Breakdown is then initiated with the conversion of the C‐3 hydroxyl group to a ketone (cholest‐4‐en‐3‐one, cholestenone) by the oxidase ChoD, and further oxidation at the C‐26 “tail” region via a three‐step process involving oxidation to the hydroxyl, aldehyde, and carboxylic acid species. These sidechain‐modifying reactions are catalysed by the cytochromes P450 CYP125A1 and CYP142A1 (CYP125 and CYP142 hereafter). Comparison of the effect of complementing a CYP125 knockout in the CDC1551 strain of Mtb (which does not express the CYP142 protein), with CYP125 or CYP142 reveals that the two enzymes are functionally redundant with respect to growth on cholesterol. Here we present a series of compounds based on an ethyl 5‐(pyridin‐4‐yl)‐1H‐indole‐2‐carboxylate pharmacophore which bind strongly to both Mtb cholesterol oxidases CYP125 and CYP142.

The introduction of a methylenecyclohexyl group on the indole NH, compound 7, maintained affinity with both CYP125 and CYP142. Upon inspection of the corresponding CYP125 ligand complex X‐ray crystals structures, it was noted that elaboration from the R1 position (N of the indole) dramatically changes the binding pose of this series. In the cases of compounds 7, 8, 10, and 12 the ligand is observed at a greater distance from the heme, typically with the pyridine coordination mediated via a water molecule, to produce a reverse‐type I interaction similar to what was observed for the inhibitor LP10. In the case of compounds 7 and 8, which feature an aliphatic ring on a methylene linker, it appears that movement of the compound deeper into the active site is blocked by Phe100, leading to a distance of 3.9 Å and 3.3 Å, respectively between the pyridine nitrogen and the heme distal water molecule. R1 position are observed significantly closer to the heme iron, with compound 10 observed at 2.4 Å from the distal water. This is likely attributable to the ability of the additional carbon to facilitate positioning of the ring closer to the plane of the indole, as opposed to compounds 7 and 8 which extend at an angle of 67° from this plane because of the geometric requirements of the single carbon linker. In the crystal structures of CYP125 in complex with 7 and 8, Ile97 and Phe100, which form part of the loop preceding the B’ helix, are positioned below the R1 ring structures seemingly blocking further ingress of the compounds. In the same structures, Thr201, which is found in the loop preceding the F α‐helix is observed in a different conformation relative to that which is observed for compound 4, forming a hydrogen bond with the sidechain of Glu271 and further restricting any downward movement of the compound.

> NGPSPNLPPGFDFTDPAIYAERLPVAEFAELRSAAPIWWNGQDPGKGGGFHDGGFWAITKLNDVKEISRHSDVFSSYENGVIPRFKNDIAREDIEVQRFVMLNMDAPHHTRLRKIISRGFTPRAVGRLHDELQERAQAIAAEAAAAGSGDFVEQVSCELPLQAIAGLLGVPQEDRGKLFHWSNEMTGNEDPEYAHIDPKASSAELIGYAMKMAEEKAKNPADDIVTQLIQADIDGEKLSDDEFGFFVVMLAVAGNETTRNSITQGMMAFAEHPDQWELYKKVRPETAADEIVRWATPVTAFQRTALRDYELSGVQIAAGQRVVMFYRSANFDEEVFQDPFTFNILRNPNPHVGFGGTGAHYCIGANLARMTINLIFNAVADHMPDLKPISAPERLRSGWLNGIKHWQVDYTGRCPVAH Diels-Alderases (DAs), functionally unique enzymes catalysing [4 + 2] cycloaddition reactions, have received considerable research interest. Our previous studies revealed that two berberine bridge enzyme (BBE)-like enzymes function sequentially in the biosynthetic pathway of D–A type natural product chalcomoracin. Unlike most BBE-like enzymes, which typically catalyze various oxidation reactions using FAD as a cofacor, such as oxidative cyclization by EcBBE20, tetrahydrocannabinolic acid synthase (THCAS), and cannabidiol acid synthase (CBDAS), and oxidative dehydrogenation by MaMO and AtBBE-like 1323, MaDA stands out because it catalyzes a non-redox intermolecular Diels–Alder reaction. Our findings suggest that these DAs have evolved from an ancestor functioning as a flavin adenine dinucleotide (FAD)-dependent oxidocyclase (OC), which catalyses the oxidative cyclisation reactions of isoprenoid-substituted phenolic compounds.

To gain insight into the structure-function relationships between OCs and DAs, we determined the crystal structure of a multifunctional Diels-Alderase MaDA1. Notably, two DAs (MaDA1 and MaDA4) and two DSs (MaDS1 and MaDS6) exhibit functional promiscuity, also functioning like OCs to produce moracin D (2). Comparative analysis of the protein structures of MaDA1, ancDA, and ancDADS revealed a similar overall fold to BBE-like enzymes, as previously reported. Specifically, they possess six β-sheets (β12-14 and β16-18), one α-helix (α11), one loop (loop in MaDA1), and a cofactor FAD, and share a similar substrate-binding pocket among these enzymes. Notably, the structural analysis also suggested the volumes of the substrate-binding pockets in ancDADS, ancDA, MaDA, and MaDA1 are similar, indicating that no significant substrate-binding pocket expansion occurred during the evolution of the standalone DAs. Enzymatic assays showed that ancDA is functionally similar to MaDA1 and MaDA4. In contrast, the transition state maintains an interaction with the active site of ancDADS-mut4 as well as ancDA and MaDA1 over the course of our simulation. Similar results were observed in the computational studies of MaDA1. Through crystal structure determination, computational calculations, and site-directed mutagenesis experiments, we identified several critical substitutions, including S348L, A357L, D389E and H418R that alter the substrate-binding mode and enable the OCs to gain intermolecular DA activity during evolution. Four substitutions, specifically S348L, A357L, D389E, and H418R, altered the binding mode of diene 3 and morachalcone A from the competitive accommodation to a simultaneous one in the enzyme, and provided the catalytic residues essential for the DA activity, resulting in the functional transition from OCs into DAs in Moraceae plants.

>[2x]MKSSFVFAKIAILLFSLVLLASANHTHEEFLQCLSSRIPKSIIYASNNPSYSNVLDSTTQNPRFLSSSTRNPSVIVTPFKISHIQPTIYCSKKHGVQIRIRSGGHDYEGLSYQSSVPFFILDLRNINSIQVDVEKKSAWVEAGATLGELYYSIAKKSKTLGFPGGLCSTVGVGGQLGGGGYGYQSRTYGLASDNIIDAQLIDARGRILNRKSMGEDLFWAIRGGGAGSFGIVIAWKVRLIDVPSTVTVFETVRMWEDNVTKKFVHRYQRRASNIDKDLTIFLGFRTTNTSDEQGNSKIQIITIISATFHGSRDRLLPLMQEEFPELGLGKEDFKEMSWVQSIVHYNNYKDDDPLEVLLNKTVNFEPNPFKLKSDYVKKPIPDDVLEKLLARLYEEDIGYDFVEFFPYGGKLSEISESEIPFPHRAGNLYNLRYMASWKQGENTTRINNHLSWVRSVYDSMTPYVSKNPRGAYLNFRDLDIGVNPNESDTTSAYNYVKQASVWGTKYFKNNFYKMVFIKTLVDPTNFFTYEQSIPPILHH> MVNISDFFGKNKKSVRSSTSRPTRQVGSSKPEVIDLDTESDQESTNKTPKKMPVSNVIDVSETPEGEKKLPLPAKRKASSPTVKPASSKKTKPSSKSSDSASNITAQDVLDKIPSLDLSNVHVKENAKFDFKSANSNADPDEIVSEIGSFPEGKPNCLLGLTIVFTGVLPTLERGASEALAKRYGARVTKSISSKTSVVVLGDEAGPKKLEKIKQLKIKAIDEEGFKQLIAGMPAEGGDGEAAEKARRKLEEQHNIATKEAELLVKKEEERSKKLAATRVSGGHLERDNV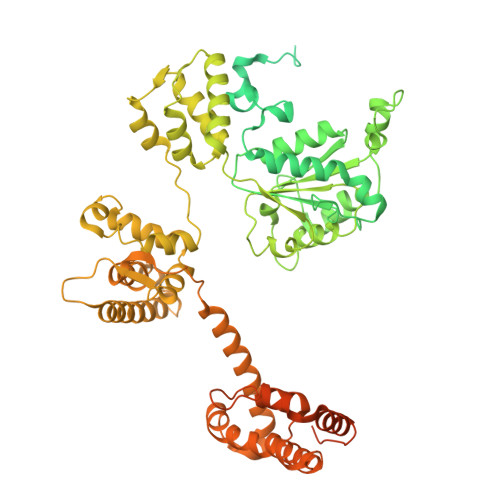REEDKLWTVKYAPTNLQQVCGNKGSVMKLKNWLANWENSKKNSFKHAGKDGSGVFRAAMLYGPPGIGKTTAAHLVAQELGYDILEQNASDVRSKTLLNAGVKNALDNMSVVGYFKHNEEAQNLNGKHFVIIMDEVDGMSGGDRGGVGQLAQFCRKTSTPLILICNERNLPKMRPFDRVCLDIQFRRPDANSIKSRLMTIAIREKFKLDPNVIDRLIQTTRGDIRQVINLLSTISTTTKTINHENINEISKAWEKNIALKPFDIAHKMLDGQIYSDIGSRNFTLNDKIALYFDDFDFTPLMIQENYLSTRPSVLKPGQSHLEAVAEAANCISLGDIVEKKIRSSEQLWSLLPLHAVLSSVYPASKVAGHMAGRINFTAWLGQNSKSAKYYRLLQEIHYHTRLGTSTDKIGLRLDYLPTFRKRLLDPFLKQGADAISSVIEVMDDYYLTKEDWDSIMEFFVGPDVTTAIIKKIPATVKSGFTRKYNSMTHPVAIYRTGSTIGGGGVGTSTSTPDFEDVVDADDNPVPADDEETQDSSTDLKKDKLIKQKAKPTKRKTATSKPGGSKKRKTKA> GAASGAKSLFSTAFSESL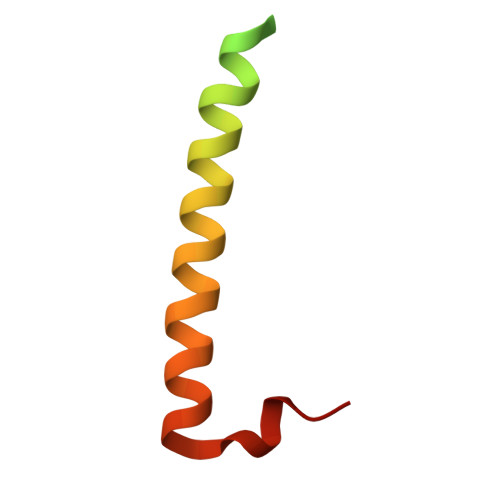AAEISSVSRDELMEAIQKQEEINFRLQDYIDRIIVAIMETNPSILEVK>GSHMATNWGSLLQDKQQLEELARQAVDRALAEGVLLRTSQEPTSSEVVSYAPFTLFPSLVPSALLEQAYAVQMDFNLLVDAVSQNAAFLEQTLSSTIKQDDFTARLFDIHKQVLKEGIAQTVFLGLNRSDYMFQRSADGSPALKQIEINTISASFGGLASRTPAVHRHVLSVLSKTKEAGKILSNNPSKGLALGIAKAWELYGSPNALVLLIAQEKERNIFDQRAIENELLARNIHVIRRTFEDISEKGSLDQDRRLFVDGQEIAVVYFRDGEMPRQYSLQNWEARLLLERSHAAKCPDIATQLAGTKKVQQELSRPGMLEMLLPGQPEAVARLRATFAGLYSLDVG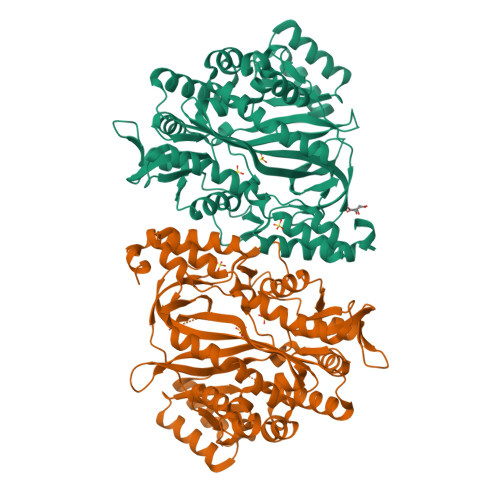EEGDQAIAEALAAPSRFVLKPQREGGGNNLYGEEMVQALKQLKDSEERASYILMEKIEPEPFENCLLRPGSPARVVQCISELGIFGVYVRQEKTLVMNKHVGHLLRTKAIEHADGGVAAGVAVLDNPYPV[2x]N-(2-MORPHOLIN-4-YL-1-MORPHOLIN-4-YLMETHYL-ETHYL)-3-NITRO-5-(3,4,5-TRIHYDROXY-6-HYDROXYMETHYL-TETRAHYDRO-PYRAN-2-YLOXY)-BENZAMIDE 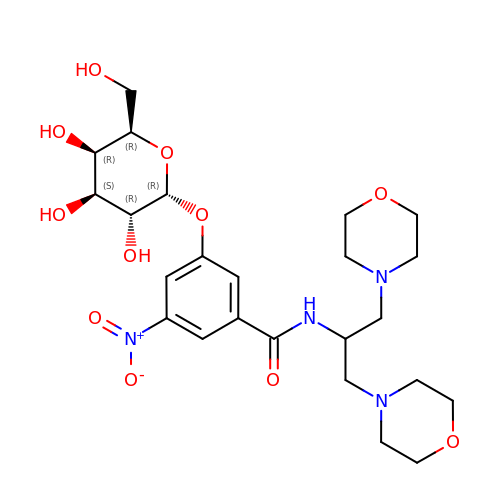| C24 H36 N4 O11 | MCMWCTMAKPQTPI-WGNYYXNJSA-N> SLAQSSPAG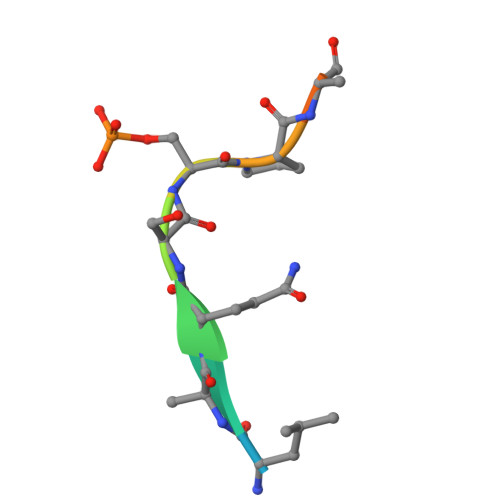SQ N-[(2R)-2-benzyl-4-(hydroxyamino)-4-oxobutanoyl]-L-alanine 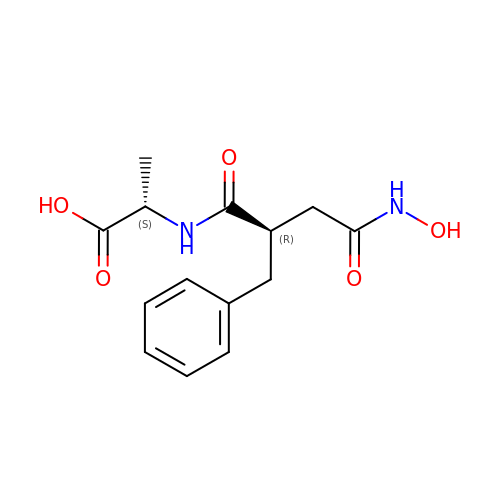| C14 H18 N2 O5 | OJCFZTVYDSKXNM-GXSJLCMTSA-N Reverse gyrase is a bacterial/archaeal type IA DNA topoisomerase that catalyzes the ATP-dependent introduction of positive supercoils into DNA. The general architecture of reverse gyrase has become evident from crystal structures of the enzymes from Archaeoglobus fulgidus and Thermotoga maritima. Both enzymes are large (>120 kDa) monomeric entities that consist of a helicase domain containing the ATP-binding site and a type IA topoisomerase domain fused on the same poly­peptide chain. The two parts of reverse gyrase, the helicase domain and the topoisomerase domain, are structurally connected by the latch, an insertion in the helicase subdomain H2. The latch couples the activity of the helicase domain to strand passage.

Here, we report the crystal structure of T. maritima reverse gyrase containing this minimal latch at 2.9 Å resolution. To gain insight into the structural basis for this differential effect on activity, we determined the crystal structure of rgyr_minlatch. Although rgyr_minlatch crystallized in a different space group, the overall structure is similar to the structure of the full-length enzyme, revealing a padlock shape. Equally small r.m.s.d. values are observed for the individual helicase domains (0.94–0.98 Å) and topoisomerase domains (0.52–0.67 Å), demonstrating that deletion of the globular domain of the T. maritima reverse gyrase latch has no significant effect on the reverse gyrase structure outside the latch. The minimal latch formed by residues 387-PSMRFSLEELIIPD-400 emanates from the H2 sub­domain and retains its short β-sheet, i.e. the first and last four residues of the sequence. In contrast to β-turns, which have a length of four residues, the loops in β-bulges consist of five or six residues, distinguished as type 1 and type 2, respectively. Typical of type 2 β-bulge loops, the minimal latch in rgyr_minlatch forms a hydrogen bond between the NH group of residue i (Phe391) and the carbonyl group of residue i + 5. The twist is a result of Phe391, the first residue in the β-bulge loop, rotating its side chain into a void that is normally occupied by Phe401. Deletion of the globular domain entails the removal of Phe401, apparently prompting Phe391 to fill the void and maintain van der Waals interactions with the methylene groups of Glu850 in the T3 region of the topoisomerase domain. Apart from Ile398 in the β-sheet, the location of which is the same in all T. maritima structures, Phe391 is the only residue that makes any interaction with the topoisomerase domain.

> MAVNSKYHHSCINCGGLNTDERNERGLPCEVCLPEDSPSDIYRALLERKTLKEYRFYHEFWNEYEDFRSFFKKKFGKDLTGYQRLWAKRIVQGKSFTMVAPTGVGKTTFGMMTALWLARKGKKSALVFPTVTLVKQTLERLQKLADEKVKIFGFYSSMKKEEKEKFEKSFEEDDYHILVFSTQFVSKNREKLSQKRFDFVFVDDVDAVLKASRNIDTLLMMVGIPEEIIRKAFSTIKQGKIYERPKNLKPGILVVSSATAKPRGIRPLLFRDLLNFTVGRLVSVARNITHVRISSRSKEKLVELLEIFRDGILIFAQTEEEGKELYEYLKRFKFNVGETWSEFEKNFEDFKVGKINILIGVQAYYGKLTRGVDLPERIKYVIFWGTPSMRFSLEELIIPDVYTYIQASGRSSRILNGVLVKGVSVIFEEDEEIFESLKTRLLLIAEEEIIEEAEANWKELVHEVEESRRRSERELTDTSRSLLIIVESPTKAETLSRFLGRASSRKERNIIVHEAVTGEGVILFTATRGHVYDLVTKGGIHGVEEENGKFVPVYNSLKRCRDCGYQFTEDRDECPVCSSKNIDDKTETLRALREISLEADEILVATDPDVEGEKISWDVTQYLLPSTRSLRRIEMHEITRYGFKKARESVRFVDFNLVKAQIVRRVQDRWIGFELSGKLQKRFGRSNLSAGRVQSTVLGWIVEREEEYKKSEKDFTLLVLENGVNLEVEGKIADDVVTVVELQEAEEEKNPLPPYTTSSALSEISQKLRLGVQEVMDILQDLFEKGFITYHRTDSTRISLEGQNVARTYLRKIGKEDIFMGRSWSTEGAHEAIRPVKPIDARELEEMIEEGLIADLTKKHLRVYELIFNRFLASQSAAVKVKKQIVTVDVDGKRMGIEQIVEILRDGWNLFVPLTVSPRFEHRTYKIKEKKFYKKHTVPLFTQASIVEEMKKRGIGRPSTYAKIVEVLFRRGYVYEDKYKRVRPTRFGVMVYSYLKERYEKYVTEETTRRLEEIMDKVERGEEDYQATLRLLYEEIKSLMEEG> ERAGPVTWVMMIACVVVFIAMQILGDQEVMLWLAWPFDPTLKFEFWRYFTHALMHFSLMHILFNLLWWWYLGGAVEKRLGSGKLIVITLISALLSGYVQQKFSGPWF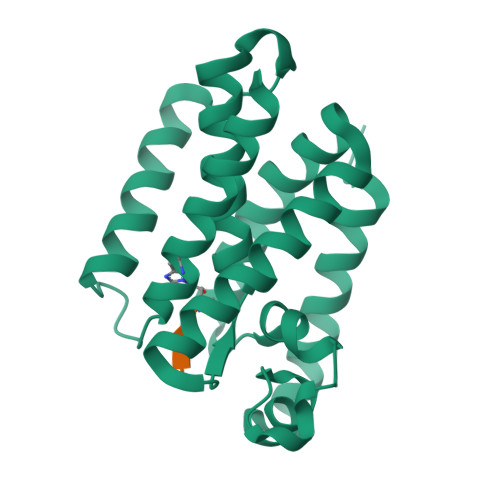GGLSGVVYALMGYVWLRGERDPQSGIYLQRGLIIFALIWIVAGWFDLFGMSMANGAHIAGLAVGLAMAFVDSLN> MVAPEHRVLHLRDRLDLAAELKLLCERGPLVRIPLEDGSAVHWFALGYDVVREVLGSEKFDKRVIGTHFNHQEMALPGNLLQLDPPEHTRLRRMVAPAFSVRRMQALEPRVQAIVDDHLDTMASTGPPVEFLREVAGPMAA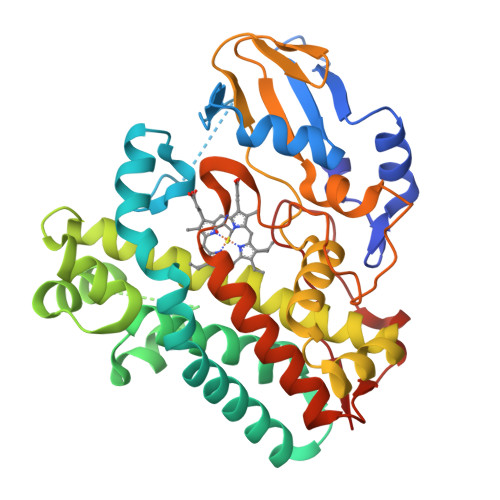RVACEFLGIPLDDRGELIRLTAHRGGKRRRVLNGHAYLAYMRELAARLRRDPGDGMLGMVARDHGADISDEELAGLCAVVMNSSVEQTESCLAAGTLLLLEHPEQFALLRERPELGEQAVEEIVRYLSVFEGLDPRTATEDVEIGGQVIKKGEAVFCSLLAANRADPALDGFDITRKESRHVAFGHGIHHCLGAPLARMELRIAFTTLVSRFPSLRTAVPAEEIRFRPPSSNVFTLLELPLTW> GSHMLRPVETPTREIKKLDGLWAFSLDRENCGIDQRWWESALQESRAIAVPGSFNDQFADADIRNYAGNVWYQREVFIPKGWAGQRIVLRFDAVTHYGKVW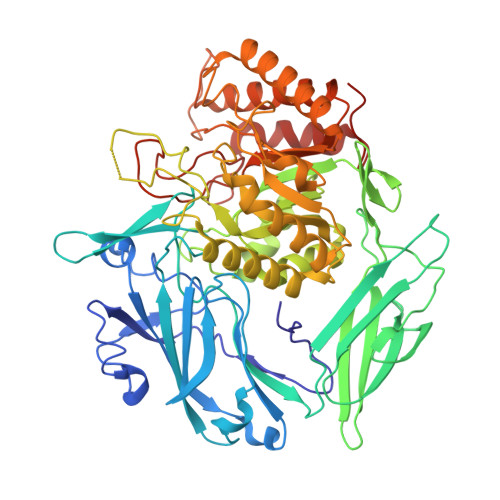VNNQEVMEHQGGYTPFEADVTPYVIAGKSVRITVCVNNELNWQTIPPGMVITDENGKKKQSYFHDFFNYAGIHRSVMLYTTPNTWVDDITVVTHVAQDCNHASVDWQVVANGDVSVELRDADQQVVATGQGTSGTLQVVNPHLWQPGEGYLYELCVTAKSQTECDIYPLRVGIRSVAVKGEQFLINHKPFYFTGFGRHEDADLRGKGFDNVLMVHDHALMDWIGANSYRTSHYPYAEEMLDWADEHGIVVIDETAAVGFNLSLGIGFEAGNKPKELYSEEAVNGETQQAHLQAIKELIARDKNHPSVVMWSIANEPDTRPQGAREYFAPLAEATRKLDPTRPITCVNVMFCDAHTDTISDLFDVLCLNRYYGWYVQSGDLETAEKVLEKELLAWQEKLHQPIIITEYGVDTLAGLHSMYTDMWSEEYQCAWLDMYHRVFDRVSAVVGEQVWNFADFATSQGILRVGGNKKGIFTRDRKPKSAAFLLQKRWTGMNFGEKPQQGGKQ> ILEAAVTQSPRNKVAVTGEKVTLSCQQTNNHNNMYWYRQDTGHGLRLIHYSYGA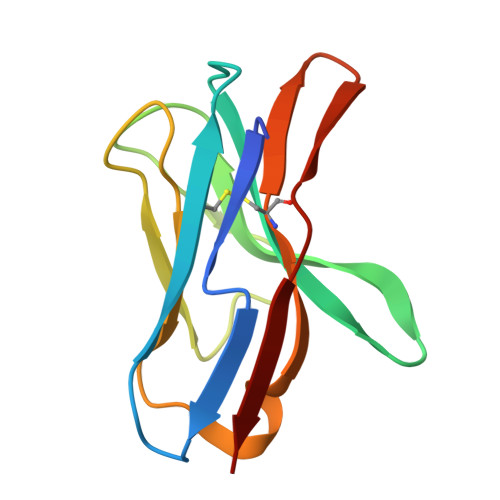GSTEKGDIPDGYKASRPSQEQFSLILESATPSQTSVYFCASGGGGTLYFGAGTRLSVL> IVGGKVCPKGECPWQVLLLVNGAQLCGGTLINTIWVVSAAHCFDKIKNWRNLIAVLGEHDLSEHDGDEQSRRVAQVIIPSTYVPGTTNHDIALLRLHQPVVLTDHVVPLCLPERTFSERTLAFVRFSLVSGWGQLLDRGATALELMVLNVPRLMTQDCEASYPGKITEYMFCAGYSDGSKDSCKGDSGGPHATHYRGTWYLTGIVSWGQGCATVGHFGVYTRVSQYIEWLQKLMRSEPRPGVLLRAPFP;> DQCASSPCQNGGSCKDQLQSYICFCLPAFEGRNCETHKDDQLICVNENGGCEQYCSDHTGTKRSCRCHEGYSLLADGVSCTPTVEYPCGKIPILEK;> TNTVAAYNLTWKSTNFKTILEWEPKPVNQVYTVQISTKSGDWKSKCFYTTDTECDLTDEI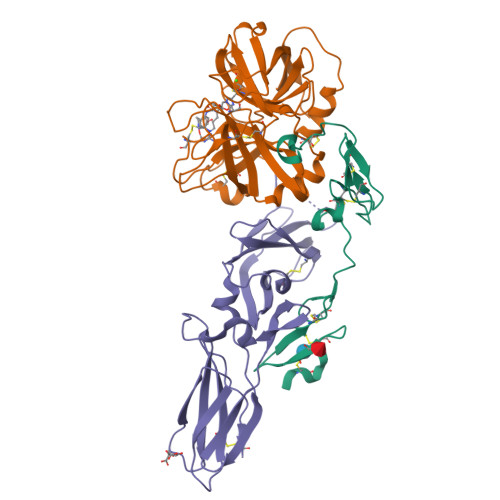VKDVKQTYLARVFSYPAGNVESTGSAGEPLYENSPEFTPYLETNLGQPTIQSFEQVGTKVNVTVEDERTLVRRNNTFLSLRDVFGKDLIYTLYYWKSSSSGKKTAKTNTNEFLIDVDKGENYCFSVQAVIPSRTVNRKSTDSPVECM Hantaviruses, a geographically diverse group of zoonotic pathogens, initiate cell infection through the concerted action of Gn and Gc viral surface glycoproteins. The ∼1,150-amino-acid glycoprotein precursor is encoded by the M segment (Schmaljohn et al., 1987) and is co-translationally cleaved by the cellular signal peptidase complex at the conserved “WAASA” sequence (Löber et al., 2001) into two structural glycoprotein components, Gn (∼70 kDa) and Gc (∼55 kDa). Low resolution three-dimensional (3D) structures of Tula (TULV) and Hantaan virus spike complexes, derived by electron cryomicroscopy studies and combined with biochemical analysis, revealed that Gn and Gc form square-shaped oligomeric complexes on the virion envelope (Battisti et al., 2011, Hepojoki et al., 2010, Huiskonen et al., 2010). Here, we describe the high-resolution crystal structure of the antigenic ectodomain of Gn from Puumala hantavirus (PUUV), a causative agent of hemorrhagic fever with renal syndrome.

Combining established techniques in cryo-ET and sub-tomogram averaging (Huiskonen et al., 2014) with direct-detector technology (Bammes et al., 2012), we improved the resolution of the TULV Gn/Gc spike structure from 36 Å (Huiskonen et al., 2010) to 16 Å. The spike complexes extend 10 nm from the 6-nm-thick viral envelope, and the membrane-distal region of the spike consists of four lobes of globular density. Consistent with the previously reported TULV structure, we observed two types of stalks linking the membrane-distal globular lobes to the virion envelope: (1) an elongated peripheral stalk that links diagonally to the membrane and cross-links with neighboring spikes and (2) a central stalk located at the center of each tetrameric spike. Computational cross-correlation-based fitting of the PUUV Gn crystal structure to the segmented cryo-ET density localized it to the four membrane-distal lobes of the spike (see Experimental Procedures). Fitting allowed identification of two alternative placements of Gn (fit A and fit B, cross-correlation coefficient 0.90–0.92) in both of the non-equivalent membrane-distal lobes (segments 1 and 2). Fitting of the PUUV Gn crystal structure into the membrane-distal part of the hantaviral spike yielded two types of solutions, A and B, with similar scoring. As these two fittings differ in the orientation of the Gn, we used additional functional constraints to discern between these two possibilities. Analyses for both of these functional constraints support fit A, as summarized below. Indeed, in our preferred fitting of PUUV Gn tetramers (fit A), we observe that the C-terminal regions of the PUUV Gn protomers co-localize toward the center of the tetrameric spike and likely contribute to the central stalk density. For our preferred PUUV Gn fitting (fit A), we observe that the N-linked glycans presented by the Gn extend from the tetrameric glycoprotein spike surface into the solvent-accessible regions between spikes.

>[2x]ETGELKIECPHTIGLGQGLVIGSVELPPVPLTQVESLKLESSCNFDLHTSTSSQQPFTKWTWEMKSDLAENTQASSTSFQTKSSEINLRGLCLVPPLVIETAARTRKTIACFDLSCNQTACQPTVFLIGPIQTCITTKSCLLGLGDQRIQVNYEKTYCVSGQLVEGVCFNPVHTMALSQPSHTYDIVTVMVRCFLIAKKVSTGDSMKLEKSFETLVQKTSCTGNGFQGYYICLVGSSSEPLYIPTLDDYRSAEVLSRMAFAPHGEDHDVEKNAISAMRIIGKVTGKAPSTESSDTIQGVAFSGNPLYTSTGVLTAKDDPVYIWAPGIIMEGNHSVCDKKTLPLTWTGFIPLPGEIEKT> EEKPKGALAVILVLTLTILVFWL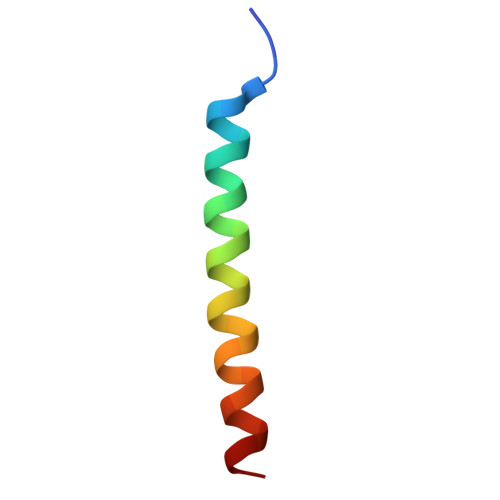GVYAVFFARG>[16x]SNAMAEDKGRKVVVSALQFACTDDVSTNVTTAERLVRAAHKQGANIVLIQELFEGYYFCQAQREDFIQRAKPYKDHPTIMRLQKLAKELGVVIPVSFFEEANNAHYNSIAIIDADGTDLGIYRKSHIP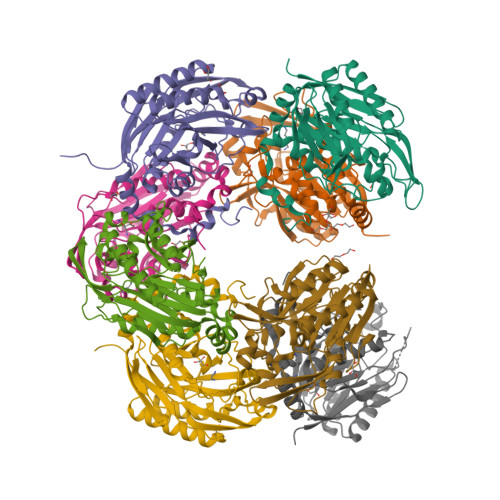DGPGYEEKFYFNPGDTGFKVFQTKYAKIGVAICWDQWFPEAARAMALQGAEILFYPTAIGSEPHDQSIDSRDHWKRVMQGHAGANLVPLVASNRIGNEIIETEHGKSEIKFYGNSFIAGPTGEIVSIADDKEEAVLIAEFNLDKIKSMRHCWGVFRDRRPDLYKVLLTLDGKNPVL> GPGSMTYQPVDITTNTIPVTKEHYYRGLELISQGKTALITPAGGQGSRLGFEHPKGMFVLPFEIPKSIFQMTSERLLRLQELASEYSHQKNVMIHWFLMTNEETIEEINNYFKEHQYFGLSSEQIHCFPQGMLPVVDF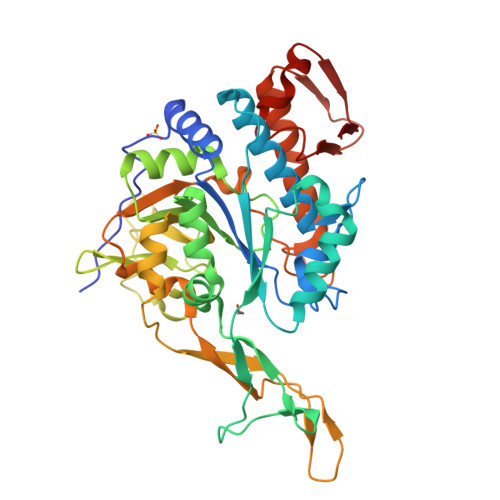NGKILYEKKDKPYMAPNGHGGLFKALKDNGILEFMNEKGIKYSVAHNVDNILCKDVDPNMIGYMDLLQSEICIKIVKKGFKEEKVGVLVKEQERIKVVEYTELTDELNKQLSNGEFIYNCGHISINGYSTSFLEKAAEYQLPYHIAKKKVPFVNEQGIVIHPSENNGIKKEIFFFDVFPLATKVSIFEIQRFIEFSALKNSLNESFDNVNTVKRDWYRLNIYYLKKAGAIVDDSKSPICEISFRKSFEEEGLKEFKGKTIQLPFILQ> GPGSMKAVNVHELAQSI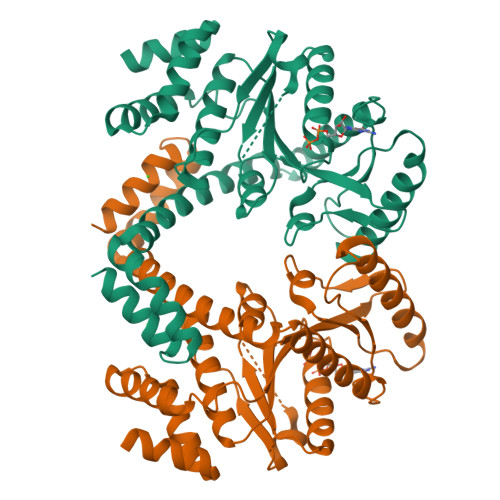RDGDRSALARAITLVESTRADHREQAQQLLLDLMPEAGSAMHVGITGVPGVGKSTTIEALGMHLIEAGHRVAVLAVDPSSTRTGGSILGDKTRMARLAVHPDAYIRPSPTSGTLGGVAKATRETIVLLEAAGYDVILVETVGVGQSEVTVAGMVDTFVFLTLARTGDQLQGIKKGVLELADVIVVNKADGEHAVEAKAAARELSGAIRLIYPRESLWRPPVLTMSAVEGTGLPELWETVLRHREVLEEAGEFEARRRTQQVEWTWSMVRDAVLDRVMNHPEVRRIRDDVEQRVRLGELTPALAAQEILDAAQ>MGSSHHHHHHSSGRENLYFSGHMIWIVGSGTCRGQTTERAKEIIERAEVIYGSRRALELAGVVDDSRARILRSFKGDEIRRIMEEGREREVAVISTGDPM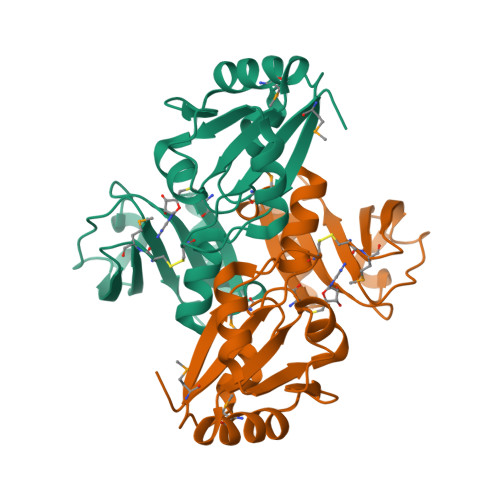VAGLGRVLREIAEDVEIKIEPAISSVQVALARLKVDLSEVAVVDCHAKDFDAELTELLKYRHLLILADSHFPLERLGKRRVVLLENLCMEGERIREGNADSIELESDYTIIFVEREVMEGS[2x]FTSJ1, a protein conserved among most eukaryotes, mediates 2’-O-methylations at position 32 (Nm32) or position 34 (Nm34), complexed with THADA or WDR6, respectively. FTSJ1 is a bifunctional protein that forms a complex with THADA (also called Trm732 in yeast) or WDR6 (also called Trm734 in yeast) to mediate Nm32 or Nm34 formation, respectively. Herein, using cryo-electron microscopy, we solve the high-resolution structure of FTSJ1-THADA with or without a tRNA substrate.

Thereafter, we incubated FTSJ1-THADA with human tRNAPhe transcripts and S-adenosyl homocysteine (SAH), followed by cryo-EM analysis. THADA forms a hollow cylindrical structure with FTSJ1 bound to the top, which completely fits the closed form of FTSJ1-THADA. Notably, the substrate tRNAPhe was located inside THADA, anchoring the anticodon loop to the methyltransferase center of FTSJ1. The interior of THADA and the tRNA binding site of FTSJ1 are strongly positively charged, facilitating the binding of the substrate tRNAPhe. The tRNA-bound FTSJ1-THADA was exclusively observed in the closed form, suggesting that THADA was stabilized in this state after tRNA binding. SAH bound to the active site of FTSJ1 via hydrogen bonds with four residues (Ser25, Ser54, Asp75, and Asp91) and several hydrophobic interactions. Moreover, the 2′-OH group of C32, the methylation target of FTSJ1-THADA, is located 3.3 Å from the sulfur atom of SAH. The THADA-binding site of FTSJ1 (Cys238-Tyr250) interacted with α62 helix and the loop between α62 and α63 of THADA, forming several hydrogen bonds, including Cys238-Pro1358, Gly239-Arg1363, Asp240-Asn1401, Ser249-Cys1393, Tyr250-Gln1400, and Tyr250-Gln1449, alongside a π–π stacking interaction of Tyr250-Phe1398. Compared to the structure of tRNA located at the P-site of the ribosome, the tRNA bound to FTSJ1-THADA exhibited a shift in the anticodon loop of approximately 10 Å. This shift, resulting from the interactions between FTSJ1-THADA and the substrate tRNAPhe, places C32 of the tRNA near the methyltransferase center of FTSJ1 and SAH. Notably, Glu1225 mutation caused a modest decrease in the methyltransferase activity of FTSJ1-THADA (lane 8), whereas other mutations in Gln680, Thr798, and Tyr843 in THADA cylindrical core and Arg199 in N-terminal tail-like domain almost completely abolished methyltransferase activity (lane 4-7).

> MDYKDDDDKSAWSHPQFEKGAENLYFQGMGVKKKKEMQVAALTICHQDLETLKSFADVEGKNLASLLLHCVQLTDGVSQIHYIKQIVPLLEKADKNGMCDPTIQSCLDILAGIYLSLSLKNPLKKVLASSLNSLPDFFLPEAMHRFTSRLQEELNTTDLYSYRKVTDNISSCMENFNLGRASVNNLLKNVLHFLQKSLIEILEENRKCAGNHIIQTQLMNDLLVGIRVSMMLVQKVQDFQGNLWKTSDSPIWQNMCGLLSIFTKVLSDDDLLQTVQSTSGLAIILFIKTMFHPSEKIPHLISSVLLRSVDCTSVPEWFMSSCRSLCCGDISQSAVLFLCQGTLAMLDWQNGSMGRSGEALLLDTAHVLFTLSSQIKEPTLEMFLSRILASWTNSAIQVLESSSPSLTDSLNGNSSIVGRLLEYVYTHWEHPLDALRHQTKIMFKNLLQMHRLTVEGADFVPDPFFVELTESLLRLEWHIKGKYTCLGCLVECIGVEHILAIDKTIPSQILEVMGDQSLVPYASDLLETMFRNHKSHLKSQTAESSWIDQWHETWVSPLLFILCEGNLDQKSYVIDYYLPKLLSYSPESLQYMVKILQTSIDAKTGQEQSFPSLGSCNSRGALGALMACLRIARAHGHLQSATDTWENLVSDARIKQGLIHQHCQVRIDTLGLLCESNRSTEIVSMEEMQWIQFFITYNLNSQSPGVRQQICSLLKKLFCRIQESSQVLYKLEQSKSKREPENELTKQHPSVSLQQYKNFMSSICNSLFEALFPGSSYSTRFSALTILGSIAEVFHVPEGRIYTVYQLSHDIDVGRFQTLMECFTSTFEDVKILAFDLLMKLSKTAVHFQDSGKLQGLFQAALELSTSTKPYDCVTASYLLNFLIWQDALPSSLSAYLTQQVACDNGDRPAAVVERNTLMVIKCLMENLEEEVSQAENSLLQAAAAFPMYGRVHCITGALQKLSLNSLQLVSEWRPVVEKLLLMSYRLSTVVSPVIQSSSPEGLIPMDTDSESASRLQMILNEIQPRDTNDYFNQAKILKEHDSFDMKDLNASVVNIDTSTEIKGKEVKTCDVTAQMVLVCCWRSMKEVALLLGMLCQLLPMQPVPESSDGLLTVEQVKEIGDYFKQHLLQSRHRGAFELAYTGFVKLTEVLNRCPNVSLQKLPEQWLWSVLEEIKCSDPSSKLCATRRSAGIPFYIQALLASEPKKGRMDLLKITMKELISLAGPTDDIQSTVPQVHALNILRALFRDTRLGENIIPYVADGAKAAILGFTSPVWAVRNSSTLLFSALITRIFGVKRAKDEHSKTNRMTGREFFSRFPELYPFLLKQLETVANTVDSDMGEPNRHPSMFLLLLVLERLYASPMDGTSSALSMGPFVPFIMRCGHSPVYHSREMAARALVPFVMIDHIPNTIRTLLSTLPSCTDQCFRQNHIHGTLLQVFHLLQAYSDSKHGTNSDFQHELTDITVCTKAKLWLAKRQNPCLVTRAVYIDILFLLTCCLNRSAKDNQPVLESLGFWEEVRGIISGSELITGFPWAFKVPGLPQYLQSLTRLAIAAVWAAAAKSGERETNVPISFSQLLESAFPEVRSLTLEALLEKFLAAASGLGEKGVPPLLCNMGEKFLLLAMKENHPECFCKILKILHCMDPGEWLPQTEHCVHLTPKEFLIWTMDIASNERSEIQSVALRLASKVISHHMQTCVENRELIAAELKQWVQLVILSCEDHLPTESRLAVVEVLTSTTPLFLTNPHPILELQDTLALWKCVLTLLQSEEQAVRDAATETVTTAMSQENTCQSTEFAFCQVDASIALALALAVLCDLLQQWDQLAPGLPILLGWLLGESDDLVACVESMHQVEEDYLFEKAEVNFWAETLIFVKYLCKHLFCLLSKSGWRPPSPEMLCHLQRMVSEQCHLLSQFFRELPPAAEFVKTVEFTRLRIQEERTLACLRLLAFLEGKEGEDTLVLSVWDSYAESRQLTLPRTEAAC;> MDYKDDDDKGAENLYFQGMGRTSKDKRDVYYRLAKENGWRARSAFKLLQLDKEFQLFQGVTRAVDLCAAPGSWSQVLSQKIGGQGSGHVVAVDLQAMAPLPGVVQIQGDITQLSTAKEIIQHFKGCPADLVVCDGAPDVTGLHDVDEYMQAQLLLAALNIATHVLKPGGCFVAKIFRGRDVTLLYSQLQVFFSSVLCAKPRSSRNSSIEAFAVCQGYDPPEGFIPDLSKPLLDHSYDPDFNQLDGPTRIIVPFVTCGDLSSYDSDRSYPLDLEGGSEYKYTPPTQPPISPPYQEACTLKRKGQLAKEIRPQDCPISRVDTFPQPLAAPQCHTLLAPEMEDNEMSCSP phosphono (2S)-2-oxidanyl-3-phosphonooxy-propanoate | C3 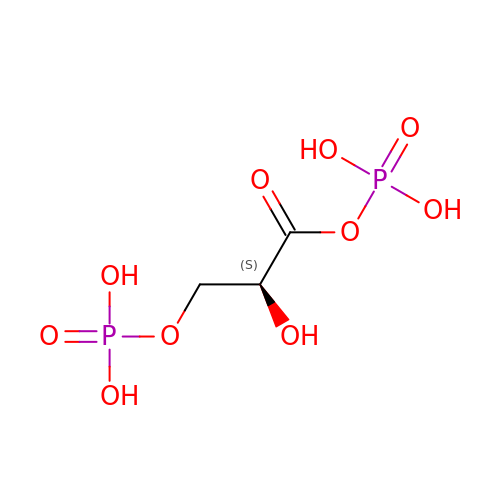H8 O10 P2 | LJQLQCAXBUHEAZ-REOHCLBHSA-N>[2x]GSGPAF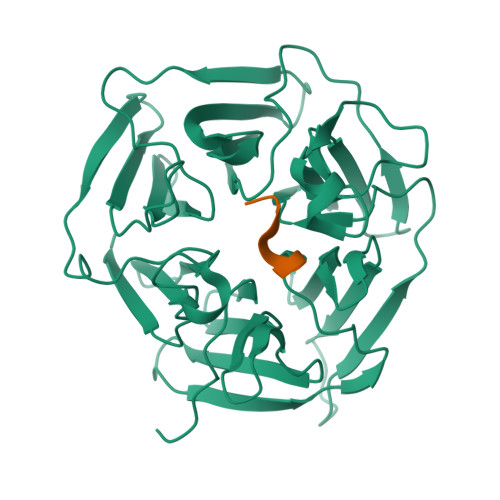ESYESMELACPAERSGHVAVSDGRHMFVWGGYKSNQVRGLYDFYLPREELWIYNMETGRWKKINTEGDVPPSMSGSCAVCVDRVLYLFGGHHSRGNTNKFYMLDSRSTDRVLQWERIDCQGIPPSSKDKLGVWVYKNKLIFFGGYGYLPEDKVLGTFEFDETSFWNSSHPRGWNDHVHILDTETFTWSQPITTGKAPSPRAAHACATVGNRGFVFGGRYRDARMNDLHYLNLDTWEWNELIPQGICPVGRSWHSLTPVSSDHLFLFGGFTTDKQPLSDAWTYCISKNEWIQFNHPYTEKPRLWHTACASDEGEVIVFGGCANNLLVHHRAAHSNEILIFSVQP;>EDSHKESNDCSCGG[2x]5'-O-(N-(L-Leucyl)-Sulfamoyl)Uridine 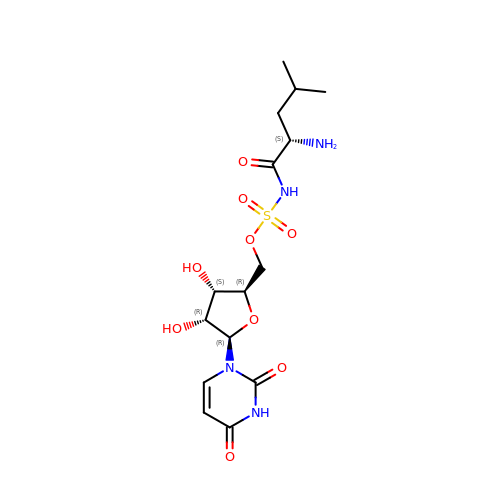| C15 H24 N4 O9 S | ZSXZGQLSAQIVTI-XKYXEJCGSA-N N-cyano-N'-[(1R)-1-phenylethyl]-N''-quinolin-5-ylguanidine | C19 H17 N5 | 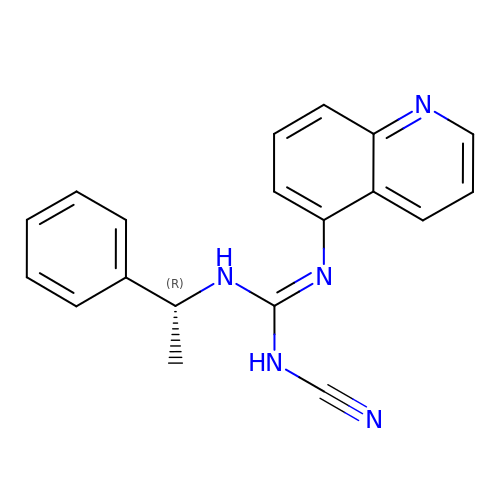PQYCRDPLPKGSME-CQSZACIVSA-N> GAEFKGLRVDMFLYNLTLQRATGISFAIHGNFSGTKQQEIVVSRGKILELLRPDPNTGKVHTLLTVEVFGVIRSLMAFRLTGGTKDYIVVGSDSGRIVILEYQPSKNMFEKIHQETFGKSGCRRIVPGQFLAVDPKGRAVMISAIEKQKLVYILNRDAAARLTISSPLEAHKANTLVYHVVGVDVGFENPMFACLEMDYEEADNDPTGEAAANTQQTLTFYELDLGLNHVVRKYSEPLEEHGNFLITVPGGSDGPSGVLICSENYITYKNFGDQPDIRCPIPRRRNDLDDPERGMIFVCSATHKTKSMFFFLAQTEQGDIFKITLETDEDMVTEIRLKYFDTVPVAAAMCVLKTGFLFVASEFGNHYLYQIAHLGDDDEEPEFSSAMPLEEGDTFFFQPRPLKNLVLVDELDSLSPILFCQIADLANEDTPQLYVACGRGPRSSLR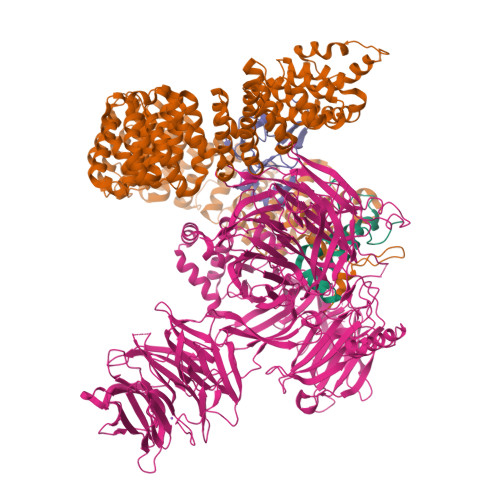VLRHGLEVSEMAVSELPGNPNAVWTVRRHIEDEFDAYIIVSFVNATLVLSIGETVEEVTDSGFLGTTPTLSCSLLGDDALVQVYPDGIRHIRADKRVNEWKTPGKKTIVKCAVNQRQVVIALTGGELVYFEMDPSGQLNEYTERKEMSADVVCMSLANVPPGEQRSRFLAVGLVDNTVRIISLDPSDCLQPLSMQALPAQPESLCIVEMGGTEKQDELGERGSIGFLYLNIGLQNGVLLRTVLDPVTGDLSDTRTRYLGSRPVKLFRVRMQGQEAVLAMSSRSWLSYSYQSRFHLTPLSYETLEFASGFASEQCPEGIVAISTNTLRILALEKLGAVFNQVAFPLQYTPRKFVIHPESNNLIIIETDHNAYTEATKAQRKQQMAEEMVEAAGEDERELAAEMAAAFLNENLPESIFGAPKAGNGQWASVIRVMNPIQGNTLDLVQLEQNEAAFSVAVCRFSNTGEDWYVLVGVAKDLILNPRSVAGGFVYTYKLVNNGEKLEFLHKTPVEEVPAAIAPFQGRVLIGVGKLLRVYDLGKKKLLRKCENKHIANYISGIQTIGHRVIVSDVQESFIWVRYKRNENQLIIFADDTYPRWVTTASLLDYDTVAGADKFGNICVVRLPPNTNDEVDEDPTGNKALWDRGLLNGASQKAEVIMNYHVGETVLSLQKTTLIPGGSESLVYTTLSGGIGILVPFTSHEDHDFFQHVEMHLRSEHPPLCGRDHLSFRSYYFPVKNVIDGDLCEQFNSMEPNKQKNVSEELDRTPPEVSKKLEDIRTRYAFDYKDDDDK;> MTDRYTIHSQLEHLQSKYIGTGHADTTKWEWLVNQHRDSYCSYMGHFDLLNYFAIAENESKARVRFNLMEKMLQPCGPPADKPEEN;> MAKIAKTHEDIEAQIREIQGKKAALDEAQGVGLDSTGYYDQEIYGGSDSRFAGYVTSIAATELEDDDDDYSSSTSLLGQKKPGYHAPVALLNDIPQSTEQYDPFAEHRPPKIADREDEYKKHRRTMIISPERLDPFADGGKTPDPKMNARTYMDVMREQHLTKEEREIRQQLAEKAKAGELKVVNGAAASQPPSKRKRRWDQTADQTPGATPKKLSSWDQAETPGHTPSLRWDETPGRAKGSETPGATPGSKIWDPTPSHTPAGAATPGRGDTPGHATPGHGGATSSARKNRWDETPKTERDTPGHGSGWAETPRTDRGGDSIGETPTPGASKRKSRWDETPASQMGGSTPVLTPGKTPIGTPAMNMATPTPGHIMSMTPEQLQAWRWEREIDERNRPLSDEELDAMFPEGYKVLPPPAGYVPIRTPARKLTATPTPLGGMTGFHMQTEDRTMKSVNDQPSGNLPFLKPDDIQYFDKLLVDVDESTLSPEEQKERKIMKLLLKIKNGTPPMRKAALRQITDKAREFGAGPLFNQILPLLMSPTLEDQERHLLVKVIDRILYKLDDLVRPYVHKILVVIEPLLIDEDYYARVEGREIISNLAKAAGLATMISTMRPDIDNMDEYVRNTTARAFAVVASALGIPSLLPFLKAVCKSKKSWQARHTGIKIVQQIAILMGCAILPHLRSLVEIIEHGLVDEQQKVRTISALAIAALAEAATPYGIESFDSVLKPLWKGIRQHRGKGLAAFLKAIGYLIPLMDAEYANYYTREVMLILIREFQSPDEEMKKIVLKVVKQCCGTDGVEANYIKTEILPPFFKHFWQHRMALDRRNYRQLVDTTVELANKVGAAEIISRIVDDLKDEAEQYRKMVMETIEKIMGNLGAADIDHKLEEQLIDGILYAFQEQTTEDSVMLNGFGTVVNALGKRVKPYLPQICGTVLWRLNNKSAKVRQQAADLISRTAVVMKTCQEEKLMGHLGVVLYEYLGEEYPEVLGSILGALKAIVNVIGMHKMTPPIKDLLPRLTPILKNRHEKVQENCIDLVGRIADRGAEYVSAREWMRICFELLELLKAHKKAIRRATVNTFGYIAKAIGPHDVLATLLNNLKVQERQNRVCTTVAIAIVAETCSPFTVLPALMNEYRVPELNVQNGVLKSLSFLFEYIGEMGKDYIYAVTPLLEDALMDRDLVHRQTASAVVQHMSLGVYGFGCEDSLNHLLNYVWPNVFETSPHVIQAVMGALEGLRVAIGPCRMLQYCLQGLFHPARKVRDVYWKIYNSIYIGSQDALIAHYPRIYNDDKNTYIRYELDYIL;> GPLGSPGSRAMAKHHPDLIFCRKQAGVAIGRLCEKCDGKCVICDSYVRPCTLVRICDECNYGSYQGRCVICGGPGVSDAYYCKECTIQEKDRDGCPKIVNLGSSKTDLFYERKKYGFKKR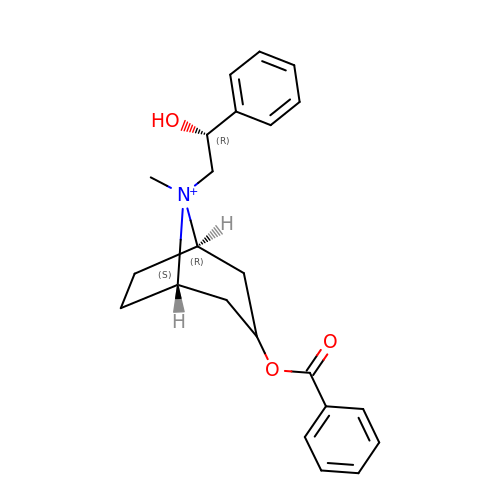[(1R,5S)-8-[(2R)-2-HYDROXY-2-PHENYL-ETHYL]-8-METHYL-8-AZONIABICYCLO[3.2.1]OCTAN-3-YL] BENZOATE | C23 H28 N O3 | UOBMQJGLFUHOEX-KVZQYWQLSA-N> AQSVPYGVSQIKAPALHSQGYTGSNVKVAVIDSGIDSSHPDLKVAGGASFVPSETNPFQDNNSHGTHVAGTVAALDNSIGVLGVAPSASLYAVKVLGADGSGQYSWIINGIEWAIANNMDVINMSLGGPSGSAALKAAVDKAVASGVVVVAAAGNEGTSGSSSTVGYPAKYPSVIAVGAVDSSNQRASFSSVGPELDVMAPGVSICSTLPGNKYGAKSGTSMASPHVAGAAALILSKHPNWT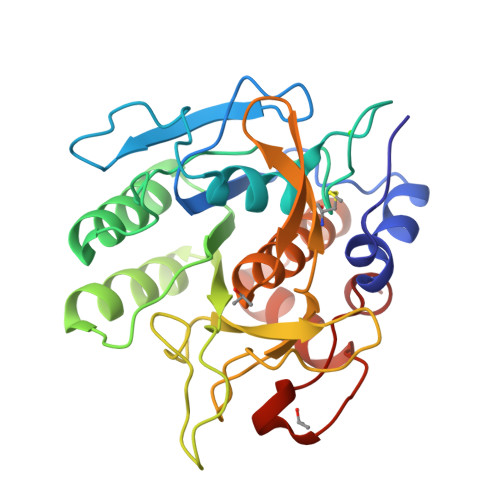NTQVRSSLENTTTKLGDSFYYGKGLINVQAAAQ Here, to gain a better understanding of fungal xylan degradation systems, which can enhance enzymatic saccharification of plant cell walls in industrial processes, we conducted a comparative study of two glycoside hydrolase family 3 (GH3) β-xylosidases (Bxls), one from the basidiomycete Phanerochaete chrysosporium (PcBxl3), and the other from the ascomycete Trichoderma reesei (TrXyl3A). The xylan main chain is degraded into xylooligosaccharides with low DPs by xylanase, and these products are further degraded into xylose by β-xylosidases (Bxls). PcBxl3 consists of three domains: (β/α)8 domain, (α/β)6-sandwich domain, and fibronectin III (FnIII)-like domain. The relationship between substrate specificity and degree of polymerization of substrates suggested that PcBxl3 preferentially degrades xylobiose (X2), while TrXyl3A degrades longer xylooligosaccharides.

The structure of PcBxl3 with xylose bound in the catalytic center was also determined. The conformation of Glu470 (PcBxl3) is the same in the native and liganded structures of PcBxl3, but Glu492 (TrXyl3A) has different conformations in native and liganded TrXyl3A. For instance, Asp267 in PcBxl3 is located at a distance of 2.7 Å from O2 of the xylose moiety bound at subsite −1, while Arg166 and Asp291 in TrXyl3A are located at distances of 2.7 Å and 2.8 Å, respectively. Glu62 and Lys183 are located at distances of 2.7 and 3.0 Å from O4 of the xylose residue in PcBxl3, respectively, and Glu89 and Lys206 in TrXyl3 are both located at a distance of 2.7 Å from O4. In addition, Trp60 of PcBxl3 and Trp87 of TrXyl3A are located near C5. The amino acids surrounding the nonreducing end sugar moiety are well conserved, but PcBxl3 has Phe129 as the residue corresponding to Tyr152 of TrXyl3A, indicating that subsite −1 of PcBxl3 would be more hydrophobic than that of TrXyl3A. In PcBxl3, there is no clearly detectable subsite +1. In the crystal structure of PcBxl3, subsite +1 was not clearly identified, but that of TrXyl3A was clearly visualized in the crystal structure.

> AFPDCANGPLKSNLVCNASADPVSRAKALVDALTLEELVNNTVNASPGVPRVGLPPYNWWSEALHGVARSPGTNFSTVPGSPFSSATSFPQPIILGATFDDDLIHSIATVISTEARAFNNAGRAGLDFFTPNINPFKDPRWGRGQETPGEDPYHIAQYVYQLITGLQGGLSPDPYYKVVADCKHFAGYDLEDWHGNNRMAFNAVISTQDLAEFYTPSFQSCVRDAHVGSVMCSYNAVNGVPSCASPYLLQDLIRDHFGLGDGWITSDCDAVDNVFDPHNYTSTLVNASAVSLKAGTDVDCGTTYSQTLVDAVNQKLVTEDDVKTSMVRLYSSLVRLGYFDSPENQPWRQLGWADVNTPSAQALALTAAEEGVVLLKNDGTLPLSRRIKHIAVVGPWANATTQMQGNYQGIAPFLISPLQALQDAGFHVSFANGTAINSTDTSGFASALMAAKAADAIVFAGGIDETIESEGHDRDSIEWPGNQLDLIEQLAALRKPLIVLQMGGGQVDSSSLKASKAVNALLWGGYPGQSGGTAIVNILTGKTAPSGRLPITQYPAAYVDAIPMTDMALRPSSSSPGRTYKWYTGTPVFDFGFGLHYTSFKLSWAASPPSRFDISSLVAGAKHAGVAFTDLAPLFTFHVAVKNSGKVTSDYVALLFAHTTVGPSPAPQQELVAYTRVKGITPGRTATAALSVTLGSIARVDESGVRSLYPGKYSVWVDTTREIMHTFELTGKTTQILGWPQPR In S. cerevisiae, the HORMAD protein Hop1 mediates the enrichment of axis proteins at nucleosome-rich islands through a central chromatin-binding region (CBR). Here, we use cryoelectron microscopy to show that the Hop1 CBR directly recognizes bent nucleosomal DNA through a composite interface in its PHD and winged helix–turn–helix domains. The Hop1 CBR comprises tightly associated PHD and winged helix–turn–helix (wHTH) domains and directly recognizes the bent DNA on nucleosomes. In S. cerevisiae, the HORMAD ortholog Hop1 contributes to axial element integrity and acts in the very early stages of meiotic recombination by mediating the recruitment of the DSB-forming endonuclease Spo11 and its accessory proteins.

We could purify the isolated S. cerevisiae Hop1 CBR (residues 322–537) but could not identify crystallization conditions. After screening the equivalent domain from several budding yeast Hop1 proteins, we determined a 1.5 Å-resolution crystal structure of the Hop1 CBR from Vanderwaltozyma polyspora (residues 317–535; 34% identical to S. cerevisiae Hop1 in this region) using single-wavelength anomalous diffraction methods (SAD) with the two natively bound zinc atoms (“Methods”). The V. polyspora Hop1 CBR structure reveals a compact assembly with a PHD domain (residues 319–374) and a variant winged helix–turn–helix (wHTH) domain (residues 375–439) with a C-terminal extension that we term HTH-C (residues 440–524). The N-terminal PHD domain coordinates two zinc ions through seven conserved cysteine residues and one conserved histidine residue. The wHTH and HTH-C domains fold together, with the HTH-C region forming an elaborated β-sheet wing on the wHTH domain and a long C-terminal ɑ-helix stretching across both the PHD and wHTH domains. Examining our structure of the V. polyspora Hop1 CBR reveals that in Saccharomycetaceae Hop1 proteins, the PHD domain’s canonical lysine binding pocket is poorly conserved and largely lacking hydrophobic residues. This lack of conservation casts doubt on whether the Hop1 PHD domain could bind a histone tail equivalently to other PHD domain proteins. Moreover, a comparison of the Hop1 CBR structure with those of DNA-bound wHTH domains reveals that in Hop1, the canonical wHTH DNA-binding surface is partially occluded by the PHD and HTH-C domains (not shown). Thus, if the Hop1 CBR directly binds nucleosome-rich chromatin as suggested by prior studies, it likely does so in a manner unlike canonical PHD or wHTH domain proteins. The overall structure of the nucleosome-bound S. cerevisiae Hop1 CBR in our cryo-EM map closely matches our crystal structure of the V. polyspora Hop1 CBR (overall Cɑ r.m.s.d. of 1.06 Å), with the most significant difference being that a disordered loop in the HTH-C domain of the V. polyspora Hop1 CBR is well-ordered and interacting with DNA in the nucleosome-bound S. cerevisiae Hop1 CBR.

> QSPDIECECDLLCPITSTRIKQCKNCRKFVHSLCYGNKPGPKVDKCISCVYGPMFDPSSSEFKDLMMLRKCYRFLSRNKGFPPSIKEFTNSIMEEGQVTLENIERINFCISTLSSDGILNFSQCNKQRDASQDGSASKATRIQGNKVSIDEEGIFVPKIGELLKGREYMCCFIYNSDNSHACYLDVSPESKRQIENWIDQVKSIRNDFEPNSS>[2x]SIQGTSLLTQSPASLSTYNDQSVSFVLENGSYVINVDDSGKDQEQDQVLLRYYESPSPASQSGDGVDGKKLMVNMSPIKDTDIWLHANDKDYSVELQRGDVSPPEQAFFVLHKKSSDFVSFESKNLPGTYIGVKDNQLALVEEKDESSNNIMFKLSKI;>ETGSKSSWGLENEALIVRCPQRGRSTYPVEWYYSDTNESIPTQKRNRIFVSRDRLKFLPARVEDSGIYACVIRSPNLNKTGYLNVTIHKKPPSCNIPDYLMYSTVRGSDKNFKITCPTIDLYNWTAPVQWFKNCKALQEPRFRAHRSYLFIDNVTHDDEGDYTCQFTHAENGTNYIVTATRSFTVEEKGFSMFPVITNPPYNHTMEVEIGKPASIACSACFGKGSHFLADVLWQINKTVVGNFGEARIQEEEGRNESSSNDMDCLTSVLRITGVTEKDLSLEYDCLALNLHGMIRHTIRLRRKHHHHHH[2x];>[2x]ET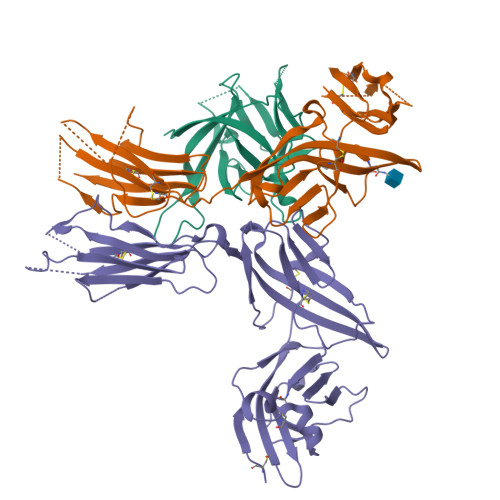GSERCDDWGLDTMRQIQVFEDEPARIKCPLFEHFLKYNYSTAHSSGLTLIWYWTRQDRDLEEPINFRLPENRISKEKDVLWFRPTLLQDTGQYTCMLRNTTYCSKVAFPLEVVQKDSCFNSAMRFPVHKMYIEHGIHKITCPNVDGYFPSSVKPSVTWYKGCTEIVDFHNVLPEGMQLSFFIPLVSNNGQYTCVVTYPENGRLFHLTRTVTVKVVGSPKDALPPQIYSPNDRVVYEKEPGEELVIPCKVYFSFIMDSHNEVWWTIDGKKPDDVTVDITINESVSYSSTEDETRTQILSIKKVTPEDLRRNYVCHARNTKGEAEQAAKVKQKHHHHHH> ATAAQAERTLPKKYGGRFTVTLIPGDGVGKEITDSVRTIFEAENIPIDWETINIKQTDHKEGVYEAVESLKRNKIGLKGLWHTPADQTGHGSLNVALRKQLDIYANVALFKSLKGVKTRIPDIDLIVIRENTEGEFSGLEHESVPGVVESLKVMTRPKTERIARFAFDFAKKYNRKSVTAVHKANIMKLGDGLFRNIITEIGQKEYPDIDVSSIIVDNASMQAVAKPHQFDVLVTPSMYGTILGNIGAALIGGPGLVAGANFGRDYAVFEPGSRHVGLDIKGQNVANPTAMILSSTLMLNHLGLNEYATRISKAVH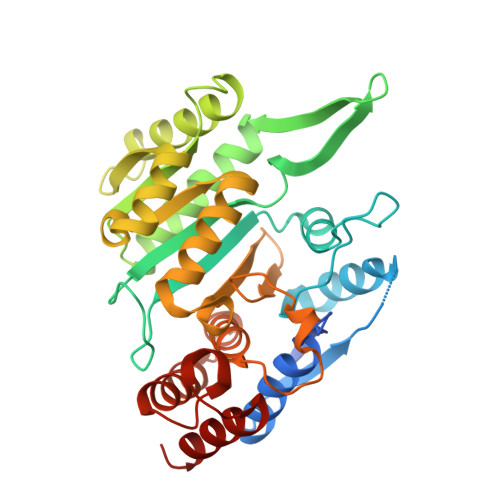ETIAEGKHTTRDIGGSSSTTDFTNEIINKLSTM>[4x]AGFCEVCKKLV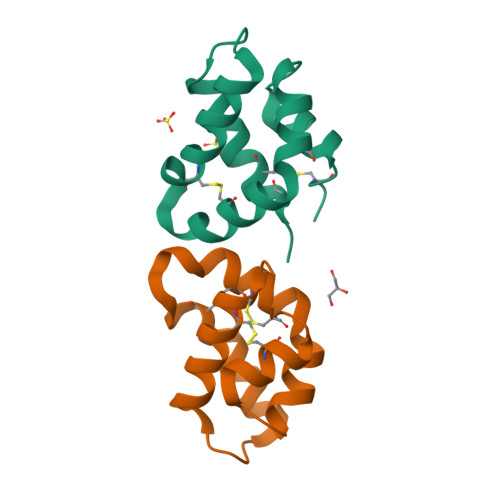GYLDRNLEKNSTKQEILAALEKGCSFLPDPYQKQCDQFVAEYEPVLIEILVEVMDPSFVCLKIGACPSHHHHHH> MRITLVTDSTSDLPQDLRGRLGVRVVPLYVNLSGAIYRDWEEITPTEIFQKVREGAAFPTTSQPSPEDFARVYREALEEADHVLSLHISGKLSGTVQSAELAA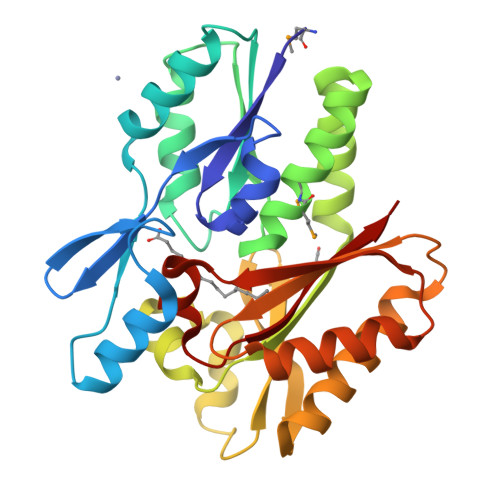QEFPGRVTVVDTQAASLGVGMMVLRAKELLEEGQSLEAVLAELERLRRDHFVRFSVATLEFLKRGGRIGGAQAFLGTLLNLKPVLTLKEGRVEAAGRARGEKKAREEILKAFRAWAEGRKRIRAYFLYSGDEDAVAALRQEVLASGLPVEEALVNELGAVIASHTGPGTYGFYAYSL>[2x]C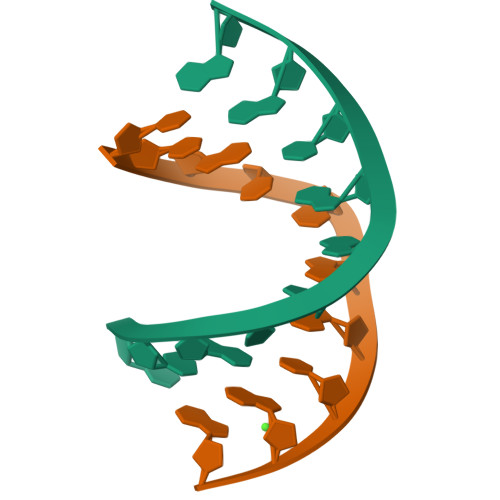CACCGGTGG> KELRCQCIKT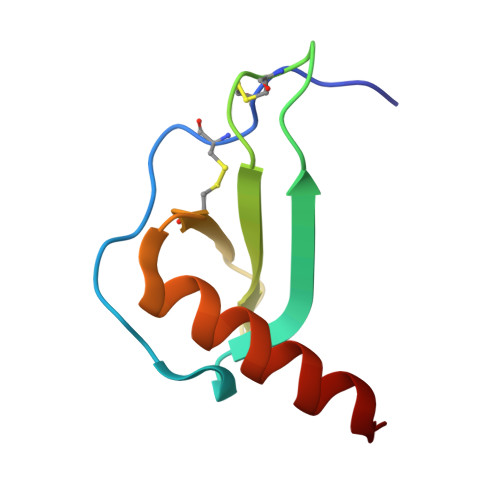YSKPFHPKFIKELRVIESGPHCANTEIIVKLSDGRELCLDPKENWVQRVVEKFLKRAENS> RKTVAKPKGPSGS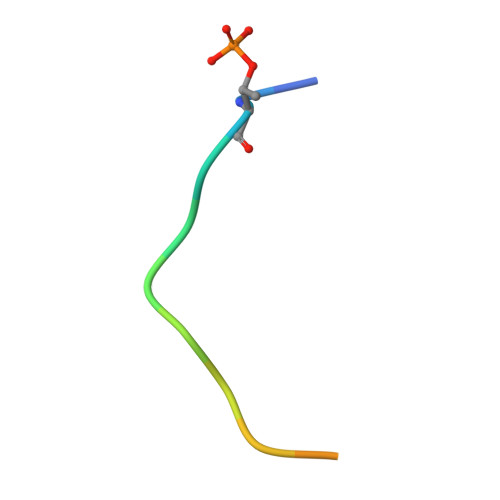PW> MNARSTGQHPARYPGAAAGEPTLDSWQEPPHNRWAFAHLGEMVPSAAVSRRPVNAPGHALARLGAIAAQLPDLEQRLEQTYTDAFLVLRGTEVVAEYYRAGFAPDDRHLLMSVSKSLCGTVVGALVDEGRIDPAQPVTEYVP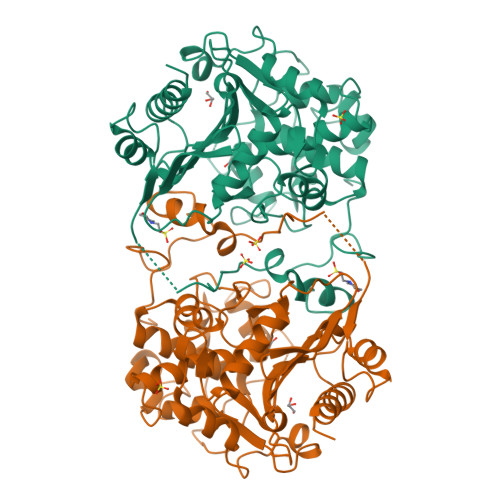ELAGSVYDGPSVLQVLDMQISIDYNEDYVDPASEVQTHGRSAGWRTRRHGDPADTYEFLTTLRGDGSTGEFQYCSANTDVLAWIVERVTGLRYVEALSTYLWAKLDADRDATITVDTTGFGFAHGGVSCTARDLARVGRMMLDGGVAPGGRVVSEDWVRRVLAGGSHEAMTDKGFTNTFPDGSYTRQWWCTGNERGNVSGIGIHGQNLWLDPLTDSVIVKLSSWPDPYTEHWHRLQNGILLDVSRALDAV> MKRLNKLLMYISSSTLLLPITLLVACTPSKVVAKPINDDEFNKLIDSIKTENDLLKYADIRFKNPNGADTKKEDIIPSQLKSENISITFKGKYQGQISAVVTNVDVDRTNPFAVQNEATIFVQFKNLKTNTSKPISITIKGLNQKGNFDASGNIVVDDFAYFGGTSGYDEYTKKDQKSRFDYDNERYMTRLKSQFGNSSNSINLKEYRGLETKQENIKKFDDQAAISNFDTYYNAALKGFTLPVYGSDGKVSGLKIYEGAEIGKGPSVVDSLGRNEKAKTVGLARTLPNEEYKTSAIQTFQTNFTIYKDYEKEIEEAEDNIKLFDSWNEQQIQSYISAQLTQLRLNYEDEVSQIDREISQTQPDKTTILSNLNQKKSKIESEYQKELSTISKLNKDSLKEWQRKEIEKYNEKKKEKTFQISESGTMWIMDYLDENAGKNPTKFYFGTNSHVAKGIKDGMVSFSLTRLNSEVKVGQTFKLNGHDSNFTKFTFSPINGNKLEDAVTAIFHATDFINENSSPLKLLDSEQKSKYNGAGIFADFAIVEVDFAKLLDKGKYSYSVWSASNDITNQYETEQNKLISKITNNYSESDKKVKFFSDSLLNEQTYAKFDRPLDFDPKKEDELKKYNDLDSLYIVGYPTAYKDFYLDQYEDEKQLKNKKYDFSLWINSEYKFYNKLINKEGSTNSFKEYETGKGNFFSYQIGYRSFIDKPGLTDAFITVNKVGKKLYS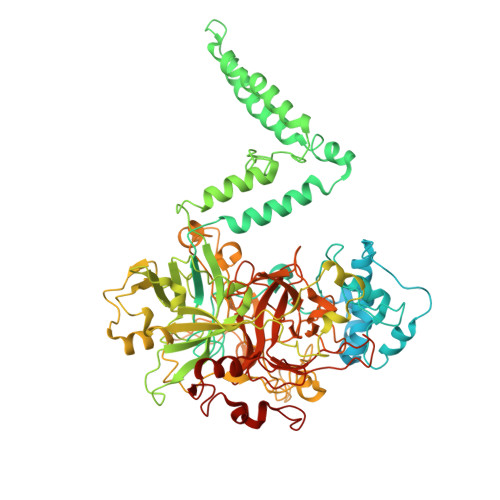LKDKNKNEVKKYFNYGLEILPRFYAPAGGASGSSVRTKDNKLLAVYHASNETARTGLAVAFRSDGYDYKNLFGDYKLGQYDLIYGGGKDQQKEKSYREVMNKMYSGKKSALFQNGFTDDKIPSEFKFNNGTQN> GSH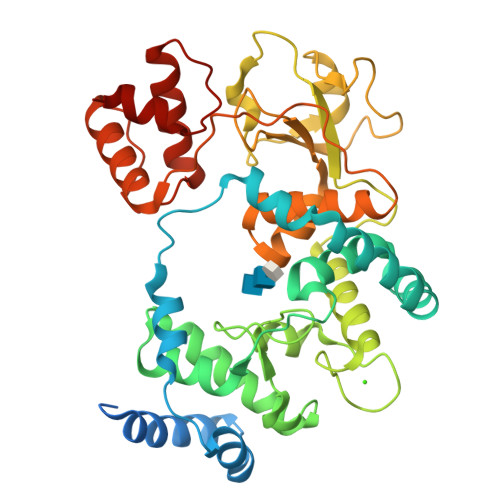MQKNPTVEYNQPAAPLQTKAPFSGAGPAASVPAGAPNEAQPGQSFEQWRDAFRQQALAGGIDAQTFDRAFAGVQPDPAVVEADRSQPEFTRPVWKYLEGALDPLRVRQGQARLAQHARILGEVDARYAVDADAVVAIWGMESNYGSHMGNKNVIRSLATLAYEGRRPEFAHAQLLAALKILQHGDVPASFMIGSWAGAMGQTQFIPTTHNQYAVDFDGDGKRDIWGSPGDALASTANYLKASGWIAGQPWGFEVRLPAGFDYSLAELTIRKPLGEWQGMGVQGVNGGPLPSGLSGEQASLLLPAGHRGPAFLVLHNFRAILKYNNSSAYALAVGLLADSFKGGGRIVGAWPLDDVPLSRSQRIELQRQLAARGHDPGAVDGIIGANTRKAIRACQQEFGWPADGYPTPALLDRLRTP>[3x]AAYSQGGGKKKVCYYYDGDIGNYYYGQGHPMKPHRIRMTHNLLLNYGLYRKMEIYRPHKA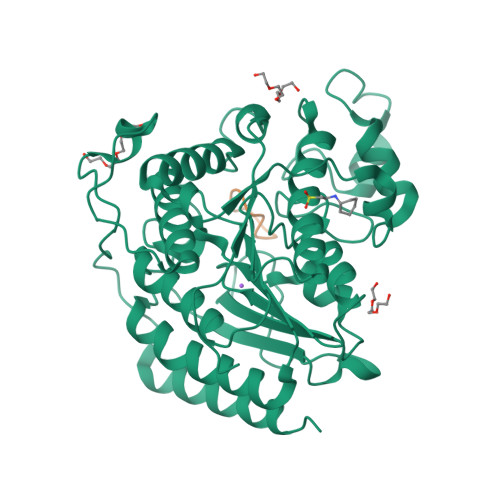TAEEMTKYHSDEYIKFLRSIRPDNMSEYSKQMQRFNVGEDCPVFDGLFEFCQLSTGGSVAGAVKLNRQQTDMAVNWAGGLHHAKKSEASGFCYVNDIVLAILELLKYHQRVLYIDIDIHHGDGVEEAFYTTDRVMTVSFHKYGEYFPGTGDLRDIGAGKGKYYAVNFPMRDGIDDESYGQIFKPIISKVMEMYQPSAVVLQCGADSLSGDRLGCFNLTVKGHAKCVEVVKTFNLPLLMLGGGGYTIRNVARCWTYETAVALDCEIPNELPYNDYFEYFGPDFKLHISPSNMTNQNTPEYMEKIKQRLFENLRMLPHAPGVQMQAI;>XWTDNSMDK[3x]>SGDRSMVEVLADHPGELVRTDSPNFLSSVLPTHWRSNKTLPIAFKVVALGDVPDGTLVTVMAGNDENYSAELRNATAAMKNQVARFNDLRFVGRSGRGKSFTLTIT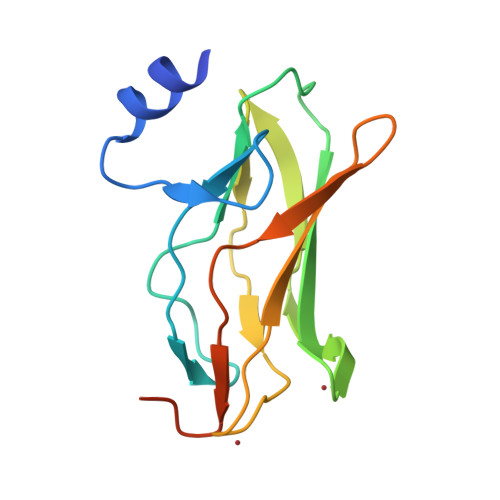VFTNPPQVATYHRAIKITVDGPREPRRHRQKLDD[2x]2-DEOXY-2-AMINO 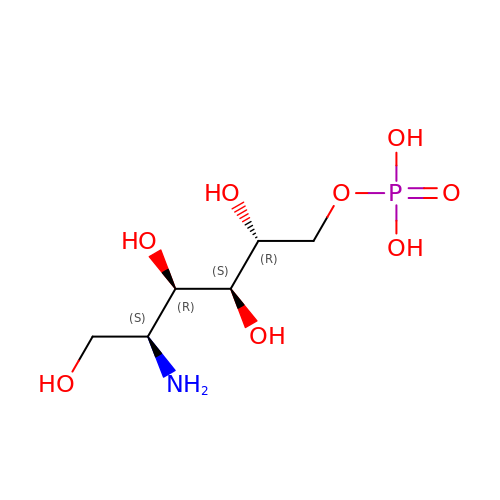GLUCITOL-6-PHOSPHATE | C6 H16 N O8 P | LBNVXZROMBUNNQ-SLPGGIOYSA-N> QDDSRYTKFLTQHYDAKPKGRDDRYCESMMVKRKLTSFCKDVNTFIHDTKNNIKAICG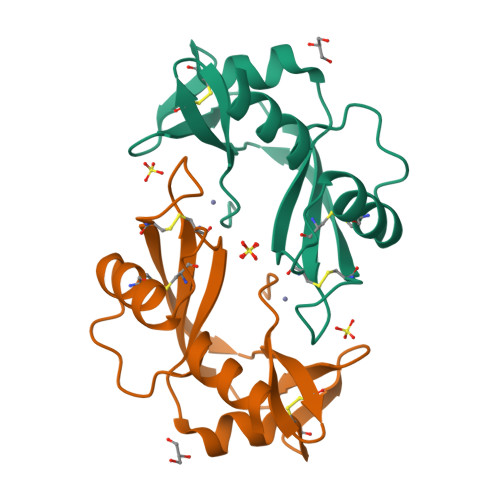KKGSPYGRNLRISKSHFQVTTCTHKGRSPRPPCRYRASKGFRYIIIGCENGWPVHFDESFISP> GSSAVNQENERLMEEYERLASELLEWIRRTIPWLENRTPEKTMQAMQKKLEDFRDYRRKHKPPKVQEKCQLEINFNTLQTKLRISNRPAFMPSEGKMVSDIAGAWQRLEQAEKGYEEWLLNEIRRLERLEHLAEKFRQKASTHETWAYGKEQILLQKDYESASLTEVRALLRKHEAFESDLAAHQDRVEQI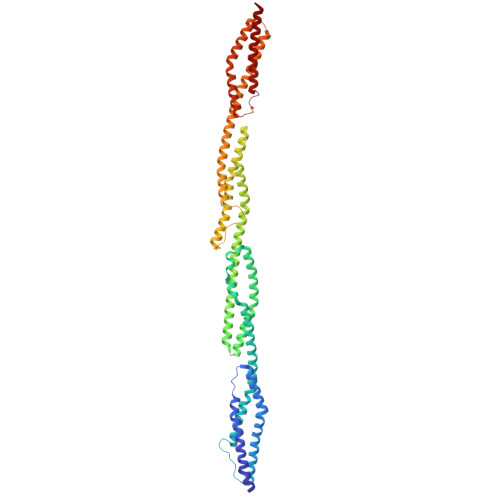AAIAQELNELDYHDAVNVNDRCQKICDQWDRLGTLTQKRREALERMEKLLETIDQLHLEFAKRAAPFNNWMEGAMEDLQDMFIVHSIEEIQSLITAHEQFKATLPEADGERQSIMAIQNEVEKVIQSYNIRISSSNPYSTVTMDELRTKWDKVKQLVPIRDQSLQEELARQHANERLRRQFAAQANAIGPWIQNKMEEIARSSIQITGALEDQMNQLKQYEHNIINYKNNIDKLEGDHQLIQEALVFDNKHTNYTMEHIRVGWELLLTTIARTINEVETQILTRD>[2x]MAAQKSPQDMDRFIDALMKKMTVEEKIGQLNLPVTGEITTGQAKSSDIAAKIKRGEVGGLFNLKGVEKIRDVQKQAVEQSRLGIPLLFGMDVIHGYETMFPIPLGLSCTWDMTAIEESARIAAIEASADGISWTFSPMVDISRDPRWGRVSEGSGEDPFLGAMIAEAMVLGYQGKDMQRN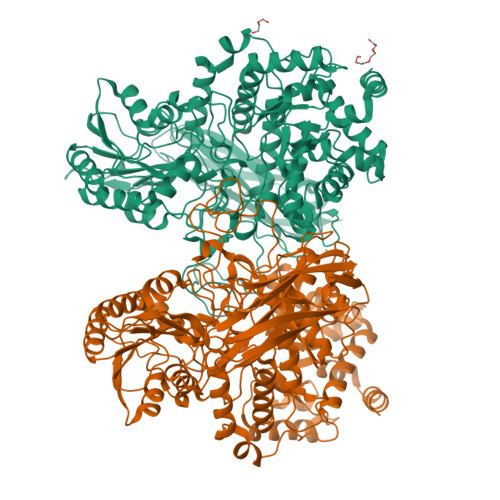DEIMACVKHFALYGAGEGGRDYNTVDMSRQRMFNEYMLPYEAAVEAGVGSVMASFNEVDGVPATANKWLMTDVLRGQWGFNGFVVTDYTGISEMIDHGIGDLQTVSARAINAGVDMDMVSEGFVSTLKKSIQEGKVSMETLNTACRRILEAKYKLGLFDNPYKYCDLKRPARDIFTKAHRDAARRIAAESFVLLKNDNVTLRPGTPAEPLLPFNPKGNIAVIGPLADSRTNMPGTWSVAAVLDRCPSLVEGLKEMTAGKANILYAKGSNLISDASYEERATMFGRSLNRDNRTDEQLLNEALTVANQSDIIIAALGESSEMSGESSSRTDLNIPDVQQNLLKELLKTGKPVVLVLFTGRPLTLTWEQEHVPAILNVWFGGSEAAYAIGDALFGYVNPGGKLTMSFPKNVGQIPLYYAHKNTGRPLAQGKWFEKFRSNYLDVDNEPLYPFGYGLSYTTFSYGDIDLSRSTIDMTGELTAAVMVTNTGTWPGSEVVQLYIRDLVGSTTRPVKELKGFQKIFLEPGQSEIVRFKIAPEMLRYYNYDLQLVAEPGEFEVMIGTNSRDVKSARFTLKLEHHHHHH> NSSTASKTYNYVYSSDPSSLNYLAENRAATSDIVANLVDGLLENDQYGNIIPSLAEDWTVSQDGLTYTYKLRKDAKWFTSEGEEYAPVTAQDFVTGLQYAADKKSEALYLVQDSVAGLDDYITGKTSDFSTVGVKALDDQTVQYTLVKPELYWNSKTLATILFPVNADFLKSKGDDFGKADPSSILYNGPFLMKALVSKSAIEYKKNPNYWDAKNVFVDDVKLTYYDGSDQESLERNFTAGAYTTARLFPNSSSYEGIKEKYKNNIIYSMQNSTSYFFNFNLDRKSYNYTSKTSDIEKKSTQEAVLNKNFRQAINFAFDRTSYGAQSEGKEGATKILR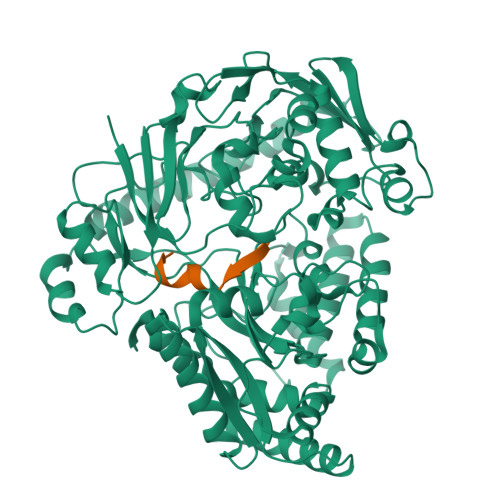NLVVPPNFVSIKGKDFGEVVASKMVNYGKEWQGINFADGQDPYYNPEKAKAKFAEAKKELEAKGVQFPIHLDKTVEVTDKVGIQGVSSIKQSIESVLGSDNVVIDIQQLTSDEFDSSGYFAQTAAQKDYDLYHGGWGPDYQDPSTYLDIFNTNSGGFLQNLGLEPGEANDKAKAVGLDVYTQMLEEANKEQDPAKRYEKYADIQAWLIDSSLVLPSVSRGGTPSLRRTVPFAAAYGLTGTKGVESYKYLKVQDKIVTTDEYAKAREKWLKEKEESNKKAQEELAKHVK;> AIQSEKARKHN> GSLIGLMKDAFQPHHHHHHHLSPHPP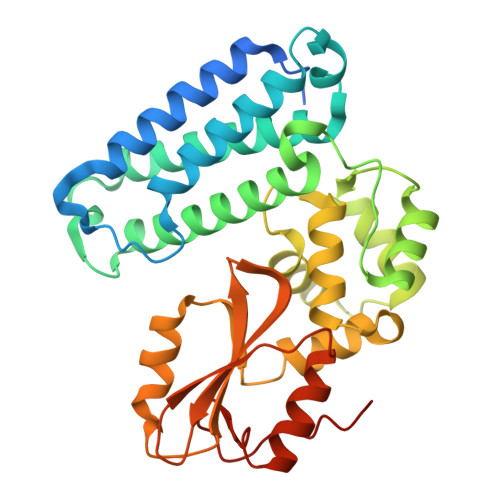GTVDKKMVEKCWKLMDKVVRLCQNPKLALKNSPPYILDLLPDTYQHLRTILSRYEGKMETLGENEYFRVFMENLMKKTKQTISLFKEGKERMYEENSQPRRNLTKLSLIFSHMLAELKGIFPSGLFQGDTFRITKADAAEFWRKAFGEKTIVPWKSFRQALHEVHPISSGLEAMALKSTIDLTCNDYISVFEFDIFTRLFQPWSSLLRNWNSLAVTHPGYMAFLTYDEVKARLQKFIHKPGSYIFRLSCTRLGQWAIGYVTADGNILQTIPHNKPLFQALIDGFREGFYLFPDGRNQNPDLTGLCEPTP>SQTVRVDIEKLDNLMDLMGELVIARSRILETLKKYNIKELDESLSHLSRITLDLQNVVMKIRMVPISFVFNRFPRMVRDLAKKMNKEVNFIMRGEDTELDRTFVEEIGEPLLHLLRNAIDHGIEPKEERIAKGKPPIGTLILSARHEGNNVVIEVEDDGRGIDKEKIIRKAIEKGLIDESKAATLSDQEILNFLFVPGFSTKEKVSEVSGRGVGMDVVKNVVESLNGSMGIESEKDKGTKVTIRLPLTLAIICALLVKVNNLVYAIPIANIDTILS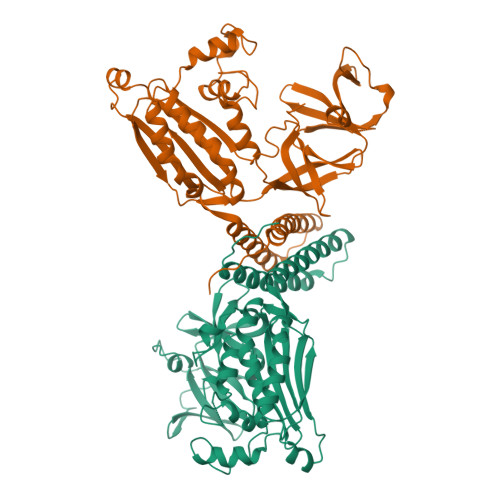ISKEDIQRVQDRDVIVIRGEVIPVYRLWEVLQIEHKEELEEMEAVIVRVGNRKYGIVVDDLLGQDDIVIKSLGKVFSEVKEFSGAAILGDGSIALIINVSGIV[2x]> QIHYSIPEEAKHGTFVGRIAQDLGLELTELVPRLFRVASKDRGDLLEVNLQNGILFVNSRIDREELCGRSAECSIHLEVIVDRPLQVFHVEVEVRDINDNPPRFPTTQKNLFIAESRPLDTWFPLEGASDADIGINAVLTYRLSPNDYFSLEKPSNDERVKGLGLVLRKSLDREETPEIILVLTVTDGGKPELTGSVQLLITVLDANDNAPVFDRSLYTVKLPENVPNGTLVVKVNASDLDEGVNGDIMYSFSTDISPNVKYKFHIDPVSGEIIVKGYIDFEECKSYEILIEGIDKGQLPLSGHCKVIVQVE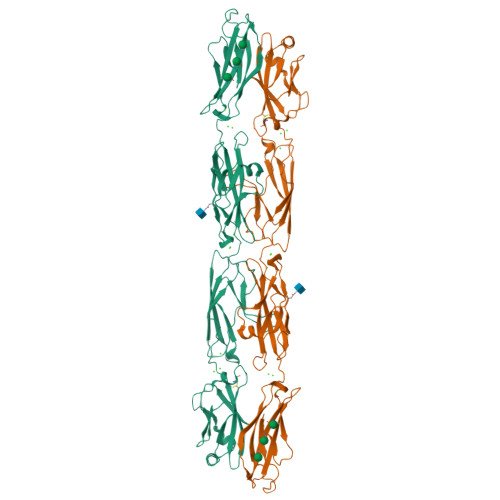DINDNVPELEFKSLSLPIRENSPVGTVIALISVSDRDTGVNGQVTCSLTSHVPFKLVSTFKNYYSLVLDSALDRETTADYKVVVTARDGGSPSLWATASVSVEVADVNDHHHHHHHH> SRHVAC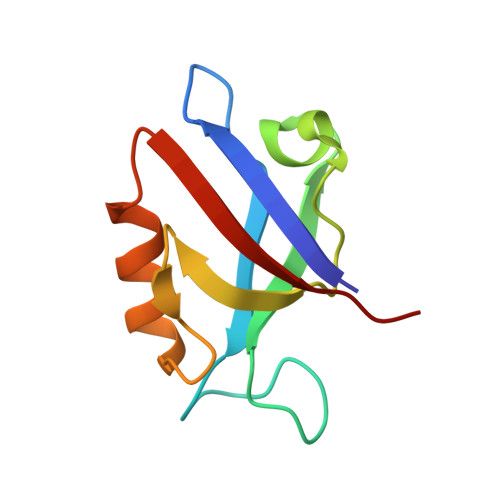LARSERGLGFSIAGGKGSTPYRAGDAGIFVSRIAEGGAAHRAGTLQVGDRVLSINGVDVTEARHDHAVSLLTAASPTIALLLEREA> 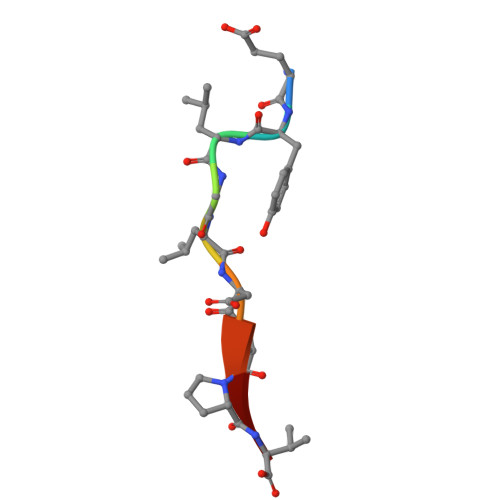EYLGLDVPV> GHMAKKTYDLLFKL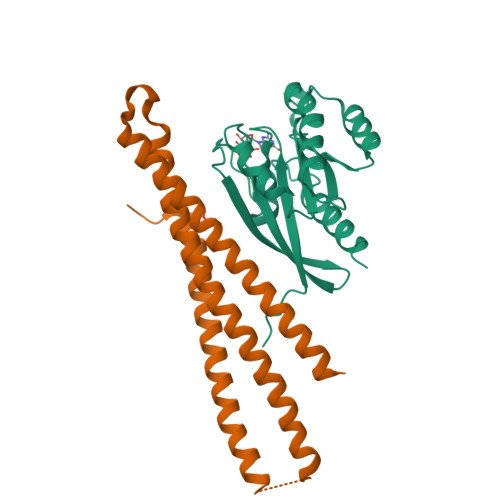LLIGDSGVGKTCVLFRFSDDAFNTTFISTIGIDFKIKTVELQGKKIKLQIWDTAGQERFHTITTSYYRGAMGIMLVYDITNGKSFENISKWLRNIDEHANEDVERMLLGNKCDMDDKRVVPKGKGEQIAREHGIRFFETSAKANINIEKAFLTLAEDILRKTPVKEPNSENVDISSGGGVTGWKSKCC;> GHMKQEELKRLYKAQAIQRQLEEVEERQRASEIQGVRLEKALRGEADSGTQDEAQLLQEWFKLVLEKNKLMRYESELLIMAQELELEDHQSRLEQKLREKMLKEESQKDEKDLNEEQEVFTELMQVIEQRDKLVDSLEEQRIREKAEDQHFES>MKTESTGKALMVLGCPESPVQIPLAIYTS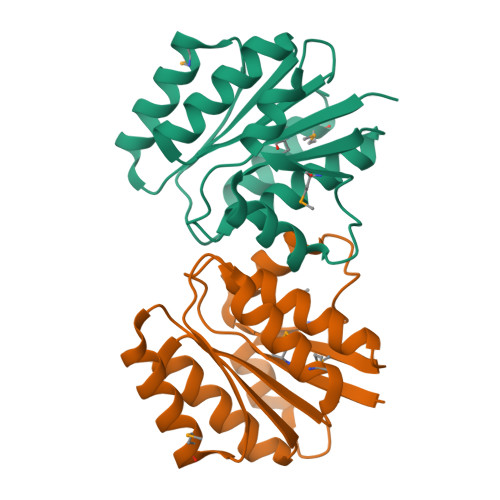HKLKKKGFRVTVTANPAALRLVQVADPEGIYTDEMVDLESCINELAEGDYEFLAGFVPNDAAAAYLVTFAGILNTETLAIIFDRDADVLEELVNEIMETLDAEIIAARAHHNPAPLRVRIDRFMEEKP[2x]>[2x]RHMASIEKVANCIRCLAADIVQGGKSGHPGTPMGMAPMSAVLWTEVMKYNSQDPDWVDRDRFVMSNGHGCALQYALLHMAGYNLTMDDLKGFRQDGSRTPGHPERFVTPGVEVTTGPLGQGIANAVGLAIAEAHLAATFNRPGYNIVDHYTYVYCGDGCLMEGVCQEALSLAGHLALEKLIVIYDSNYISIDGSTSLSFTEQCHQKYVAMGFHVIEVKNGDTDYEGLRKALAEAKATKGKPKMIVQTTTIGFGSSKQGTEKVHGAPLGEEDIANIKAKFGRDPQKKYDVDDDVRAVFRMHIDKCSAEQKAWEELLAKYTAAFPAEGAAFVAQMRGELPSGWEAKLPTNSSAIATRKASENCLAVLFPAIPALMGGSADLTPSNLTRPASANLVDFSSSSKEGRYIRFGVREHAMCAILNGLDAHDGIIPFGGTFLNFIGYALGAVRLAAISHHRVIYVATHDSIGVGEDGP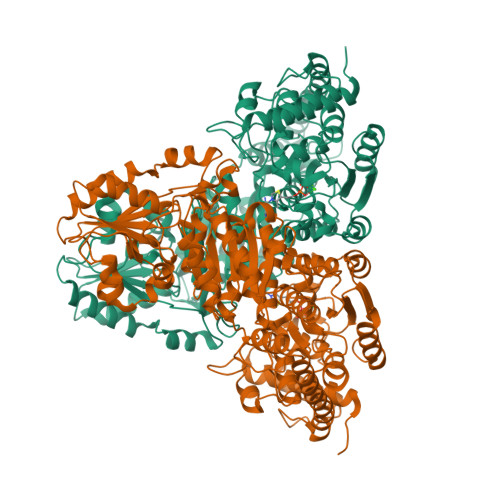THQPVELVAALRAMPNLQVIRPSDQTETSGAWAVALSSIHTPTVLCLSRQNTEPQSGSSIEGVRHGAYSVVDVPDLQLVIVASGSEVSLAVDAAKALSGELRVRVVSMPCQELFDAQPDTYRQAVLPAGVPVVSVEAYVSFGWEKYSHAHVGMSGFGASAPAGVLYKKFGITVEEVVRTGRELAKRFPDGTAPLKNSSFSKM We identified ScRIPK, a member of the RLCK VII subfamily, by a screen for sugarcane orthologs of Arabidopsis RIPK and rice GUDK. Thus, ScRIPK is a member of the RLCK VII subfamily localized in the plasma membrane. Furthermore, bacterial growth was measured to determine the bacterial proliferation inside plants, showing that transgenic plants exhibited significantly higher bacterial proliferation than that in wild-type plants at 3 days. These results suggest that ScRIPK plays role in regulating drought tolerance and disease defense in Arabidopsis. Like the typical structure of protein kinases, ScRIPK-KD contains a small N-lobe, composed of five β-sheets and an α-helix, and a large C-lobe, composed of six helices, an activation loop, and a catalytic loop.

In the ScRIPK-KD-ATP complex structure, Y169 and E170–M172 formed a deep cavity to clamp the adenine group of ATP and a magnesium ion bond with the catalytic base D237 and the β- and γ-phosphates of the nucleotide. Other residues, including G99–G101, K124, Q132, S176, K179, K221, and S223, may contribute to the stabilization of the nucleotide through hydrogen bonding. The catalytic spine is completed by the adenine base of ATP, which binds to the V103 (from the beginning of the β2-strand), A122 (from the conserved Ala-Xxx-Lys of the β3-strand), and L226 (from the middle of the C-lobe β2-strand). We also analyzed the ScRIPK-KD activation loopresidues that mediated the kinase functions. This activation loop contains three phosphorylation sites, namely, T250, S253, and T254, as indicated by the electron density. The ScRIPK kinase domain adopted an active conformation with a salt-bridge formed between K124 and E140, similar to the active conformation of other kinase proteins, such as IRAK-4, BAK1, and BRI1. In addition, we determined the location of the DFG-Phe residue and calculated its distance from two conserved residues (K124 and L144, labeled as D2 and D1, respectively) in the N-terminal domain, revealing that it belongs to the DFGin group. By analyzing the Ramachandran region annotation (A, B, L, and E) for the X, D, and F residues of the ScRIPK X-DFG motif and the DFG-Phe χ1 rotamer, we found that the ScRIPK-KD structure was in the BLAminus cluster. Furthermore, the regulatory spine (R-spine), which determines the positioning of the protein substrates so that catalysis occurs, was assembled in the ScRIPK-KD structure. The R-spine contained residues from the activation segment and the αC-helix, which assembled by the L155 (from the beginning of the β4-strand), L144 (from the C-terminal end of the αC-helix), F238 (from the activation segment conserved DFG motif), along with H/YRD-Tyr217 of the catalytic loop.

> MGSSHHHHHHSQGSMSLVGSNLHVFTIAELRAVTRDFSMTNFIGEGGFGPVYKGYVHDKTKPGLAAQTVAVKLLDLEGGQGHTEWQTEVFFLGQLRHPHLVKLIGYCYEDEHRLLVYEFMTRGSLEKHLFKKYAASLPWSTRLKIAIGAAKGLAFLHEAEKPVIYRDFKTSNILLDSDYKAKLSDFGLAKDGPEDDETHVSTRVMGTQGYAAPEYIMTGHLTAKSDVYGYGVVLLELLSGRKAVDKTRPPREQSLVEWARPYLTDARRLDRVMDPSLAGQYSTRAAHKAAAVAHQCVALNPKSRPHMSAVVDALEPLLALDDCIVG> PTMLQDWYNSQGFIGYQACAIISQHWLVDKACSMSGEDAARNGWELKSDGRKLSDEQSALIARRDMEFRVKDNLVELNRFKNVFGVRIALFVVESDDPDYYEKPFNPDGVTPGSYKGISQIDPYWAMPQLTAGSTADPSSEHFYEPDFWIISGKKYHRSHLVVVRGPQPPDILKPTYIFGGIPLTQRIYERVYAAERTANEAPLLAMSKRTSTIHVDVEKAIANEEAFNA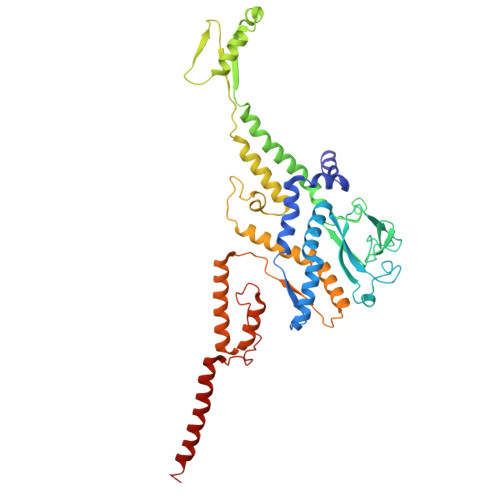RLAFWIANRDNHGVKVLGIDEGMEQFDTNLADFDSIIMNQYQLVAAIAKTPATKLLGTSPKGFNATGEHETISYHEELESIQEHIFDPLLERHYLLLAKSEEIDVQLEIVWNPVDSTSSQQQAELNNKKAATDEIYINSGVVSPDEVRERLRDDPRSGYNRLTDDQAETEPGMSPENLAEFEKAGAQSAKAKGEAERAEAQAG> SVALVPHVGMGLE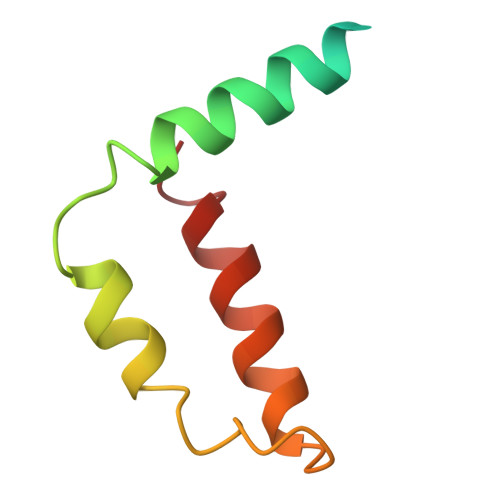TRTETWMSSEGAWKHAQRIETWILRHPGFTIMAAILAYTIGTTHFQRVLIFILLTAIAPSMT>MGMMKKTITLLTALLPLASAIAEEPTLSPAMVSAAEVVSAQENQTYTYVRCWYRTSHSKDDAATDWKWAKNQDGSDFTIDGYWWSSVSFKNMFYTNTSQNVIRQRCEETLDLANENADITFFAADNRYSYNHTIWSNDAAMQPDQINKVVALGDSLSDTGNIFNASQWRFPNPNSWFLGHFSNGFVWTEYVAKAKNLPLYNWAVGGAAGENQYIALTGVGEQVSSYLTYTKLAKNYNPANTLFTLEFGLNDFMNYNRSVPEVKADYAEALIRLTDAGAKNFMLMTLPDATKAPQFKYSTQEEIETIRAKVLKMNEFIKAQAMYYKAQGYNIALFDTHALFEKLTSAPEEHGFVNASDPCLDINRSSSVDYMYTHSLRSECAASGADKFVFWDVTHPTTATHRYVAEKMLESSNNLEEFRFHHHHHH[2x]

Vibrio dual lipases/transferases (VDLTs, e.g., VPA0226 of Vibrio parahaemolyticus, lec/VC_A0218 of Vibrio cholera, and VvPlpA of Vibrio vulnificus) are a class of virulence factors secreted by Vibrio pathogens to disrupt host membrane structures. VDLTs contain an N-terminal domain (NTD) of unknown function and a C-terminal catalytic domain belonging to the SGNH/GDSL hydrolase family, which is named after the four characteristic catalytic residues (Ser, Gly, Asn, and His). Therefore, VDLTs are enzymes with unusual dual substrate and catalytic promiscuity, which could benefit pathogens in handling diverse host lipid molecules in a proper manner. Crystal structures of the VDLT from Vibrio alginolyticus (ValDLT) and its fatty acid complexes were solved, revealing prominent structural flexibility.

We also solved the structures of ValDLT in complex with arachidonic acid (ARA) and docosahexaenoic acid (DHA), two other long-chain fatty acids (LCFAs) that can be transferred to cholesterol. ARA and DHA are buried slightly deeper in the acyl-binding pocket than OLA due to their longer hydrocarbon chains, and in general, the two complexes share similarity with ValDLT/OLA in active site conformation and ligand interactions. The hydrocarbon tails of OLA, ARA, and DHA, which are unsaturated long-chain fatty acids, all adopt a bent conformation to occupy a large portion of the pocket. Their tails follow a similar tracking path with certain differences in zigzag detail, and their carboxyl groups are in the same position with similar orientation. All three LCFA-bound structures suggest that ValDLT catalyzes substrates with long acyl chains via a different conformational pathway from those with short or medium acyl chains.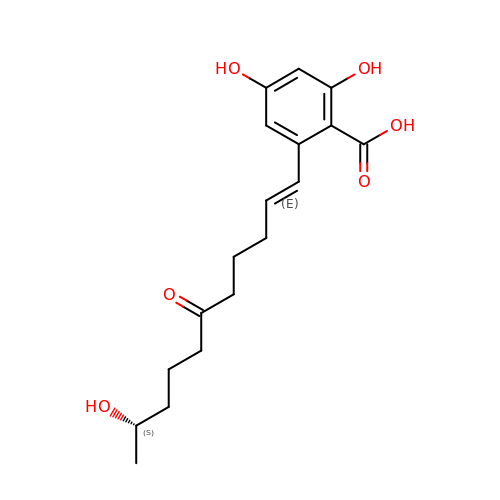2,4-dihydroxy-6-[(1E,10S)-10-hydroxy-6-oxoundec-1-en-1-yl]benzoic acid | C18 H24 O6 | KZABMNZGZHPCFB-QBODLPLBSA-N> GPGSMSRVPISEEQAQQMVAKQQAQQERMEALEEQKENMLRAFVSAEGRERLKRIAQVKAGRSQAVEMHIIQAVQRGKMQPPVSDDTVRELLGQMAN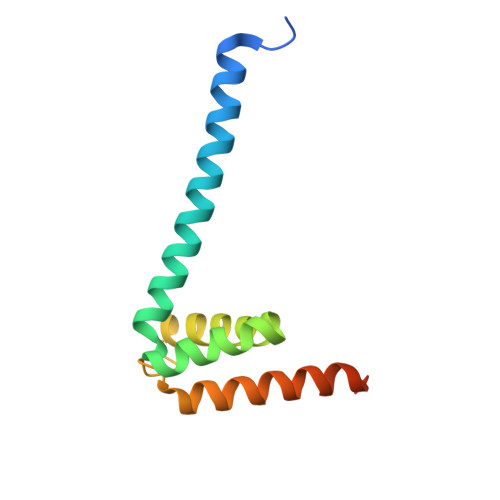QEAESRSHITIARKRTDDDW>[6x]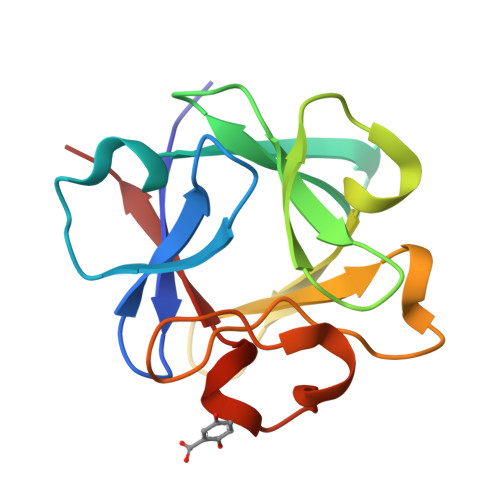KKPKLLYCSNGGHFLRILPDGTVDGTRDRSDQHIQLQLSAESVGEVYIKSTETGQYLAMDTDGLLYGSQTPNEECLFLERLEENHYNTYISKKHAEKNWFVGLKKNGSCKRGPRTHYGQKAILFLPLPVS> MTEDLFGD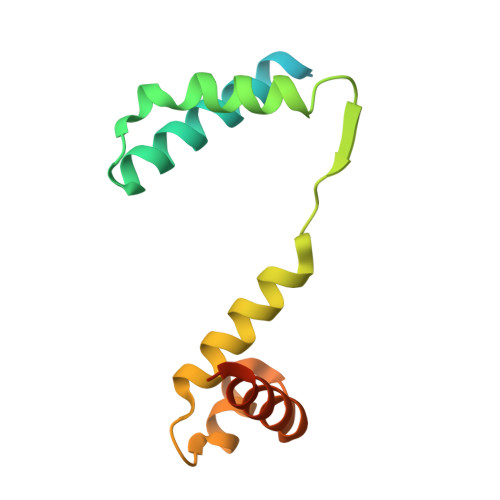LQDDTILAHLDNPAEDTSRFPALLAELNDLLRGELSRLGVDPAHSLEIVVAICKHLGGGQVYIPRGQALDSLIRDLRIWNDFNGRNVSELTTRYGVTFNTVYKAIRRMRRLKYRQYQPSLL>IGTGFPFDPHYVEVLGERMHYVDVGPRDGTPVLFLHGNPTSSYVWRNIIPHVAPTHRCIAPDLIGMGKSDKPDLGYFFDDHVRFMDAFIEALGLEEVVLVI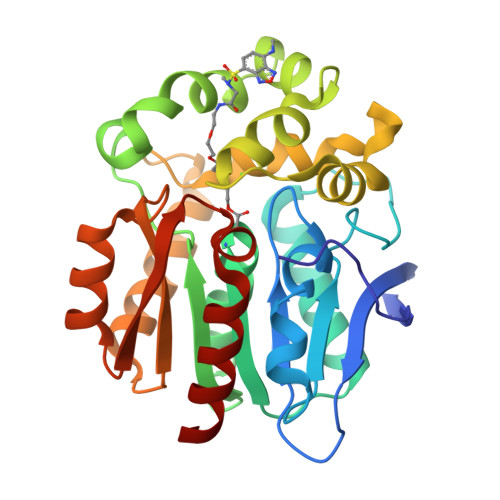HDWGSALGFHWAKRNPERVKGIAFMEFIRPIPTWDEWPEFARETFQAFRTTDVGRKLIIDQNVFIEGTLPMGVVRPLTEVEMDHYREPFLNPVDREPLWRFPNELPIAGEPANIVALVEEYMDWLHQSPVPKLLFWGTPGVLIPPAEAARLAKSLPNCKAVDIGPGLNLLQEDNPDLIGSEIARWLSTL[2x]>MKAINIALDGPAAAGKSTIAKRVASELSMIYVDTGAMYRALTYKYLKLNKTEDFAKLVDQTTLDLTYKADKGQCVILDNEDVTDFLRNNDVTQHVSYVASKEPVRSFAVKKQKELAAEKGIVMDGRDIGTVVLPDADLKVYMIASVEERAERRYKDNQLRGIESNFEDLKRDIEARDQYDMNREISPLRKADDAVTLDTTGKSIEEVTDEILAMV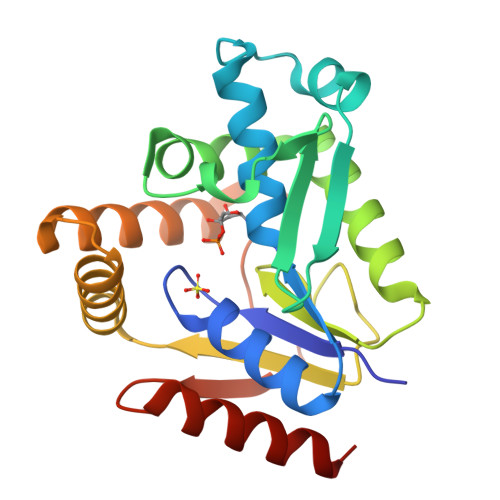SQIK[3x]> ISPI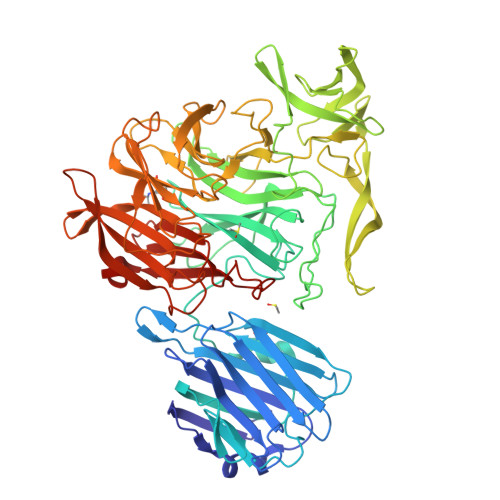FQGGSYQLNNKSIDISSLLLDKLSGESQTVVMKFKADKPNSLQALFGLSNSKAGFKNNYFSIFMRDSGEIGVEIRDAQKGINYLFSRPASLWGKHKGQAVENTLVFVSDSKDKTYTMYVNGIEVFSETVDTFLPISNINGIDKATLGAVNREGKEHYLAKGSIDEISLFNKAISDQEVSTIPLSNPFQLIFQSGDSTQANYFRIPTLYTLSSGRVLSSIDARYGGTHDSKSKINIATSYSDDNGKTWSEPIFAMKFNDYEEQLVYWPRDNKLKNSQISGSASFIDSSIVEDKKSGKTILLADVMPAGIGNNNANKADSGFKEINGHYYLKLKKNGDNDFRYTVRENGVVYNETTNKPTNYTINDKYEVLEGGKSLTVEQYSVDFDSGSLRERHNGKQVPMNVFYKDSLFKVTPTNYIAMTTSQNRGESWEQFKLLPPFLGEKHNGTYLCPGQGLALGSSNRLIFATYTSGELTYLISDDSGQTWKKSSASIPFKNATAEAQMVELRDGVIRTFFRTTTGKIAYMTSRDSGETWSKVSYIDGIQQTSYGTQVSAIKYSQLIDGKEAVILSTPNSRSGRKGGQLVVGLVNKEDDSIDWKYHYGIDLPSYGYAYSAITELPNHHIGVLFEKYDSWSRNELHLSNVVQYIDLEINDLT> MSPILGYWKIKGLVQPTRLLLEYLEEKYEEHLYERDEGDKWRNKKFELGLEFPNLPYYIDGDVKLTQSMAIIRYIADKHNMLGG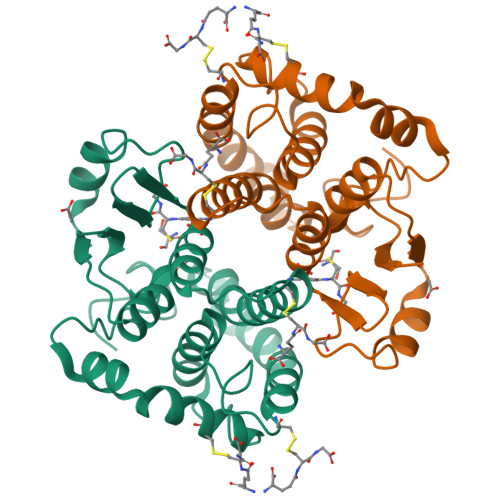CPKERAEISMLEGAVLDIRYGVSRIAYSKDFETLKVDFLSKLPEMLKMFEDRLCHKTYLNGDHVTHPDFMLYDALDVVLYMDPMCLDAFPKLVCFKKRIEAIPQIDKYLKSSKYIAWPLQGWQATFGGGDHPPKSGSYSYSY>[4x]GMLPDDVNQADVLADVTAAFYRYEKALTGNDVAVLDELFWHDEKTVRYGAGENLYGIE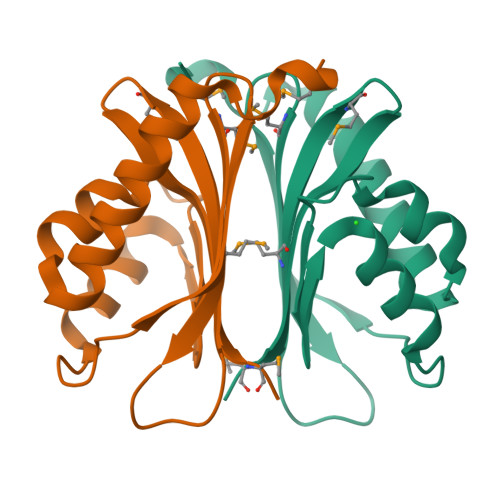EIRAFRLARPSAGLDRALRNTVITTYGHDMAVASTEFTRTGSTKIGRQMQTWVKMPEGWRIVAAHVSLMSE> PGGVPWIAIGDETSVTSPGALRRMTSKDIPETAIINTDNSSGAVPSESALVPYNDEPLVVVTEHAIANFTKAEMALEFNREFLDKLRVLSVSPKYSDLLTYVDCYVGVSARQALNNFQKQVPVITPTRQTMYVDSIQAALKALEKWEIDLRVAQTLLPTNVPIGEVSCPMQSVVKLLDDQLPDDSLIRRYPKEAAVALAKRNGGIQWMDVSEGTVMNEAVNAVAASALAPSASAPPLEEKSKLTEQAMDLVTAAEPEIIASLVPVPAPVFAIPPKPADYNVRTLKIDEATWLRMIPKTMGTLFQIQVTDNT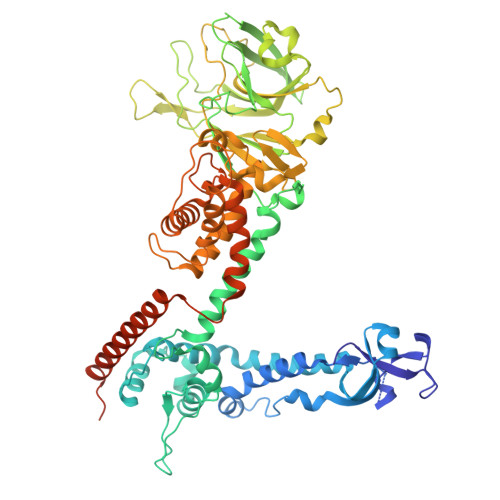GTNWHFNLRGGTRVVNLDQIAPMRFVLDLGGKSYKETSWDPNGKKVGFIVFQSKIPFELWTAASQIGQATVVNYVQLYAEDSSFTAQSIIATTSLAYNYEPEQLNKTDPEMNYYLLATFIDSAAITPTNMTQPDVWDALLTMSPLSAGEVTVKGAVVSEVVPAELIGSYTPESLNASLPNDAARCMIDRASKIAEAIKIDDDAGPDEYSPNSVPIQGQLAISQLETGYGVRIFNPKGILSKIASRAMQAFIGDPSTIITQAAPVLSDKNNWIALAQGVKTSLRTKSLSAGVKTAVSKLSSSESIQNWTQGFLDKVSTHFPAPKPDCPTNGDGSEPSARRVKRDSYAGVVKRGYTR Native single-wavelength anomalous dispersion (SAD) is an attractive experimental phasing technique as it exploits weak anomalous signals from intrinsic light scatterers (Z < 20). Here, the benefit of using a wavelength of 2.7 over 1.9 Å is demonstrated for native-SAD phasing on a 266 kDa multiprotein-ligand tubulin complex (T2R-TTL) and is applied in the structure determination of an 86 kDa helicase Sen1 protein at beamline BL-1A of the KEK Photon Factory, Japan. In this work, performed at beamline BL-1A at the Photon Factory with two real-life targets T2R-TTL and Sen1, we have demonstrated that the increased anomalous signal at 2.7 Å (sulfur f′′ = 1.5 e−) over shorter wavelengths can be harnessed effectively as long as the crystal dimension in the beam path is smaller than 100 µm, and extra material around the crystal and air scattering are minimized. Both Sen1 and T2R-TTL can diffract to about 2.4 Å resolution, but only data up to 3 Å were collected and successfully used for phasing.

We applied native-SAD measurement using a wavelength of 2.7 Å on Sen1: an 85.7 kDa helicase protein with 32 S atoms, involved in the termination of non-coding transcription processes. The Sen1 crystal measured as 220 × 100 × 50 µm was carefully mounted on an elliptical loop with minimum surrounding solvent [Fig. 3(a)]. We then successfully applied a 2.7 Å wavelength to solve a 86 kDa helicase Sen1 protein using a multi-orientation data-collection protocol.

> MNSAELAKQELEHMRKRLNVDMNPLYEIILQWDYTRNSEYPDDEPIGNYSDVKDFFNSPADYQKVMKPLLLLESWQGLCSSRDREDYKPFSIIVGNRTAVSDFYDVYASVAKQVIQDCGISESDLIVMAYLPDFRPDKRLSSDDFKKAQHTCLAKVRTLKNTKGGNVDVTLRIHRNHSFSKFLTLRSEIYCVKVMQMTTIEREYSTLEGLEYYDLVGQILQAKPSPPVNVDAAEIETVKKSYKLNTSQAEAIVNSVSKEGFSLIQGPPGTGKTKTILGIIGYFLSTKNASSSNVIKVPLEKNSSNTEQLLKKQKILICAPSNAAVDEICLRLKSGVYDKQGHQFKPQLVRVGRSDVVNVAIKDLTLEELVDKRIGERNYGSGSKNSVNYRNRDLDRRNAQAHILAVSDIICSTLSGSAHDVLATMGIKFDTVIIDEACQCTELSSIIPLRYGGKRCIMVGDPNQLPPTVLSGAASNFKYNQSLFVRMEKNSSPYLLDVQYRMHPSISKFPSSEFYQGRLKDGPGMDILNKRPWHQLEPLAPYKFFDIISGRQEQNAKTMSYTNMEEIRVAIELVDYLFRKFDNKIDFTGKIGIISPYREQMQKMRKEFARYFGGMINKSIDFNTIDGFQGQEKEIILISCVRADDTKSSVGFLKDFRRMNVALTRAKTSIWVLGHQRSLAKSKLWRDLIEDAKDRSCLAYACSGFLDPRNNRAQSILRKFNVPVPSEQEDDYKLPMEYITQGPDEVKSN~{S}-[2-[3-[[(2~{R})-4-[[[(2~{S},3~{R},4~{S},5~{R})-5-(6-aminopurin-9-yl)-4-oxidanyl-3-phosphonooxy-oxolan-2-yl]methoxy-oxidanyl-phosphoryl]oxy-oxidanyl-phosphoryl]oxy-3,3-dimethyl-2-oxidanyl-butanoyl]amino]propanoylamino]ethyl] 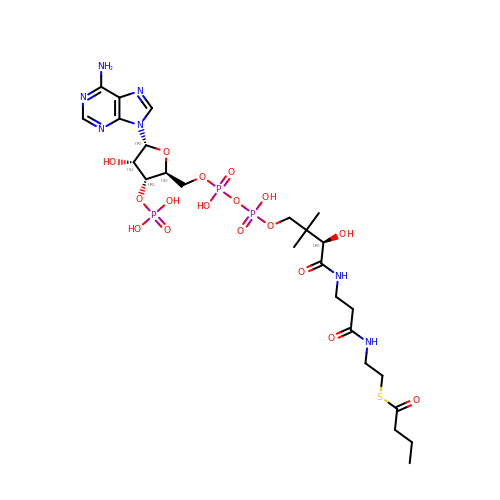butanethioate | C25 H42 N7 O17 P3 S | CRFNGMNYKDXRTN-JSFVJHESSA-N3-aminopropane-1-sulfonic acid | C3 H9 N O3 S | 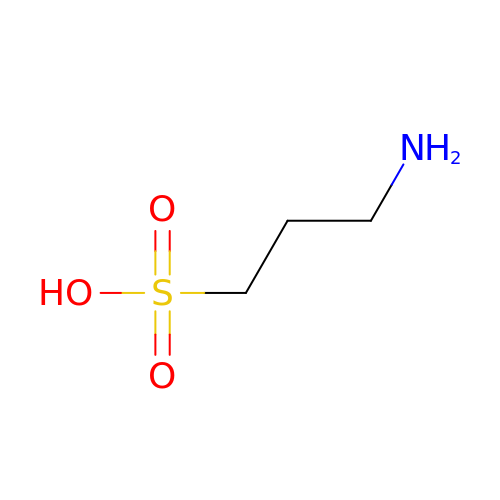SNKZJIOFVMKAOJ-UHFFFAOYSA-N> WNRNPSARYPKKGNKGCRPV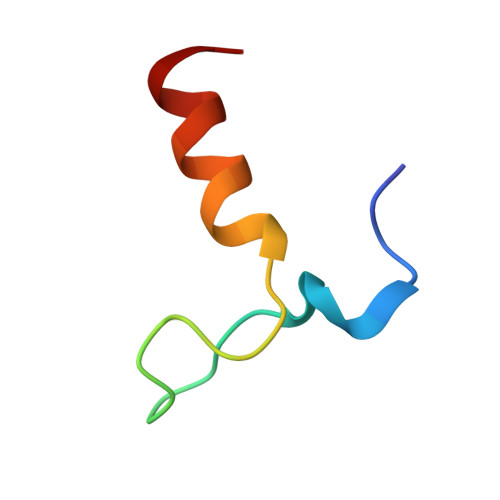CRAMRKIRKRLRTGR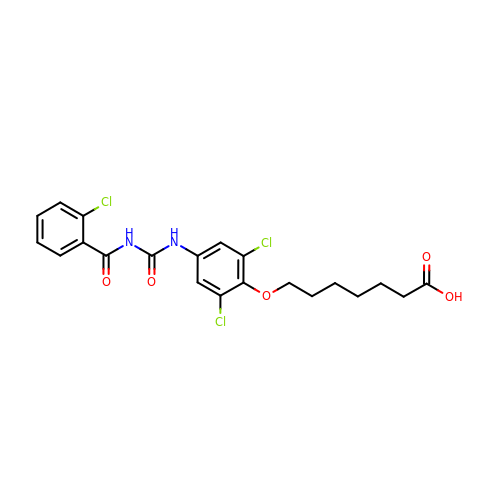7-[2,6-DICHLORO-4-({[(2-CHLOROBENZOYL)AMINO]CARBONYL}AMINO)PHENOXY]HEPTANOIC ACID | C21 H21 Cl3 N2 O5 | XQTOWNDCHQJXOQ-UHFFFAOYSA-N> GGSMKIKEVIVVEGKDDTAAIRRAVDADTIETNGAAVGAEVIERIKLAKERRGVIIFTDPDFPGE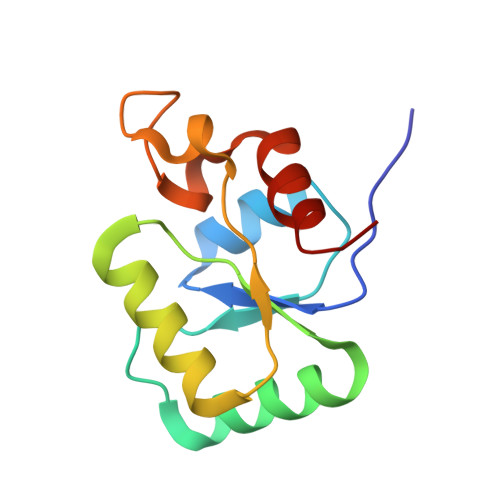KIRRTIAEQVPGCKHAFLPREAAKARSGKGIGVEHASPDDIRQALANVYEE> GSHMSNAKTKLGITKYSIVTNSNDSVTLRLMTEHDLAMLYEWLNRSHIVEWWGGEEARPTLADVQEQYLPSVLAQESVTPYIAMLNGEPIGYAQSYVALGSGDGWWEEETDPGVRGIDQLLANASQLGKGLGTKLVRALVELLFNDPEVTKIQTDPSPSNLRAIRCYEKAGFERQGTVTTPDG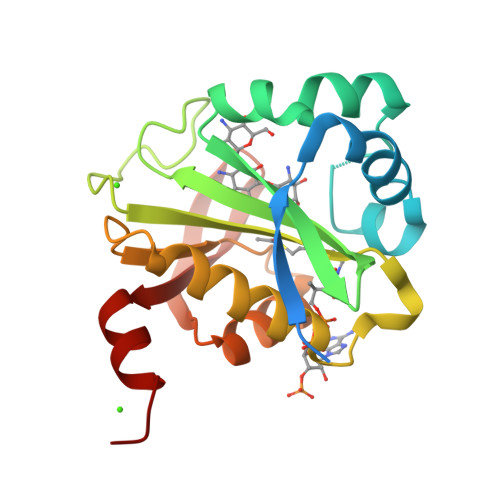PAVYMVQTRQAFERTRSDA> 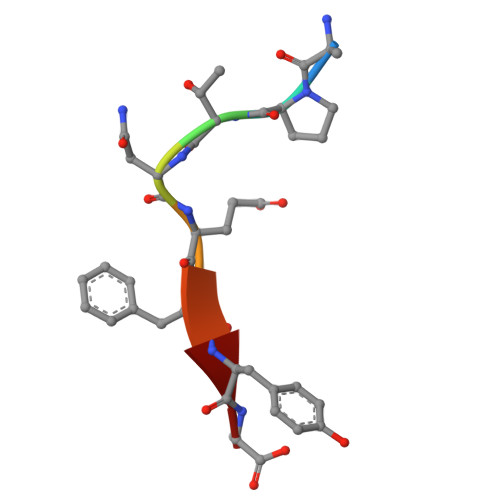APTNEFYA Protein nanocages attracted intense attention as drug delivery systems due to their high biocompatibility, high solubility, and ease of surface modification. Among proteins, a special position is occupied by the ferritin superfamily since it has been shown that these proteins can selectively deliver anticancer drugs to cancer cells. Arsenoplatin-1 ([Pt(µ-NHC(CH3)O)2ClAs(OH)2]), also called AP-1, is the most representative member of this class. As the ferritin (Ft) nanocage has already been used to encapsulate a variety of metallodrugs, we explore here whether it is an appropriate nanocarrier for AP-1.

The AP-1-encapsulated horse spleen apo-ferritin (AFt) was prepared following the alkaline pH procedure previously reported for cisplatin-encapsulated AFt. Briefly, the protein cage is disassembled at basic pH and then reassembled in the presence of a large amount of the metallodrug (a protein subunit to AP-1 molar ratio of 1:50 was used). AP-1-encapsulated AFt was then crystallized and X-ray diffraction data on these crystals were collected at 1.50 Å at high resolution at ESRF synchrotron in Grenoble, France. The overall structure of AP-1-encapsulated AFt, reported in Figure 4A, is very similar to that of the metal-free protein. Root mean square deviation between the carbon alpha atoms of each protein chain is as low as 0.13 Å. Upon reaction with the protein, an AP-1 fragment that has lost the chloride ligand binds the side chain of His49 retaining the Pt-As bond. The Pt(II) center coordinates the ND1 atom of the histidine side chain; the Pt-ND1 distance is 2.5 Å. The AP-1 fragment forms hydrogen bonds with the side chain of Glu53 and with solvent molecules. One of the OH groups bound to As interacts with the side chain of Arg52 and with a water molecule. Since more than one molecule of AP-1 per AFt chain is present, analysis of the protein structure points out that there are a lot of free AP-1 molecules trapped within the bulk.

> SSQIRQNYSTEVEAAVNRLVNLYLRASYTYLSLGFYFDRDDVALEGVCHFFRELAEEKREGAERLLKMQNQRGGRALFQDLQKPSQDEWGTTLDAMKAAIVLEKSLNQALLDLHALGSAQADPHLCDFLESHFLDEEVKLIKKMGDHLTNIQRLVGSQAGLGEYLFERLTLK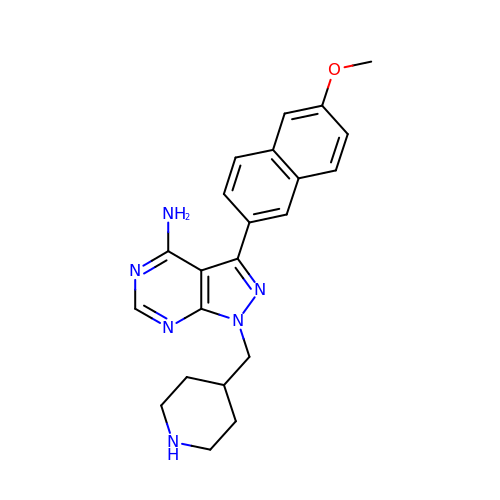3-(6-methoxynaphthalen-2-yl)-1-(piperidin-4-ylmethyl)-1H-pyrazolo[3,4-d]pyrimidin-4-amine | C22 H24 N6 O | MBHHJCMRPHUOAD-UHFFFAOYSA-N>[8x]MRQETRFKFNAYLSRVAEL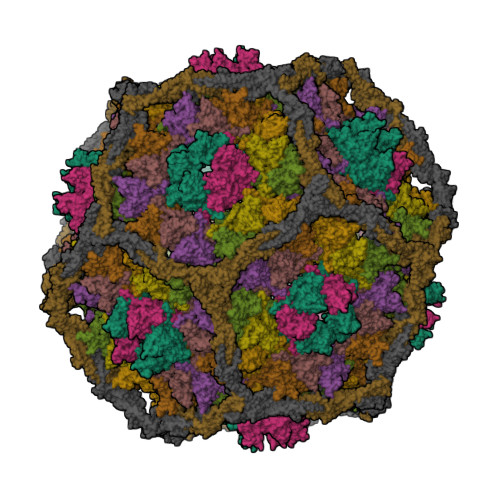NGIDAGDVSKKFTVEPSVTQTLMNTMQESSDFLTRINIVPVSEMKGEKIGIGVTGSIASTTDTAGGTERQPKDFSKLASNKYECDQINFDFYIRYKTLDLWARYQDFQLRIRNAIIKRQSLDFIMAGFNGVKRAETSDRSSNPMLQDVAVGWLQKYRNEAPARVMSKVTDEEGRTTSEVIRVGKGGDYASLDALVMDATNNLIEPWYQEDPDLVVIVGRQLLADKYFPIVNKEQDNSEMLAADVIISQKRIGNLPAVRVPYFPADAMLITKLENLSIYYMDDSHRRVIEENPKLDRVENYESMNIDYVVEDYAAGCLVEKIKVGDFSTPAKATAEPGA;>[2x]MSDHTIPEYLQPALAQLEKARAAHLENARLMDETVTAIERAEQEKNALAQADGNDADDWRTAFRAAGGVLSDELKQRHIERVARRELVQEYDNLAVVLNFERERLKGACDSTATAYRKAHHHLLSLYAEHELEHALNETCEALVRAMHLSILVQENPLANTTGHQGYVAPEKAVMQQVKSSLEQKIKQMQISLTGEPVLRLTGLSAATLPHMDYEVAGTPAQRKVWQDKIDQQGAELKARGLLS>SMRKKIFKPEELRQALMPTLEALYRQDPESLPFRQPVDPQLLGIPDYFDIVKNPMDLSTIKRKLDTGQYQEPWQY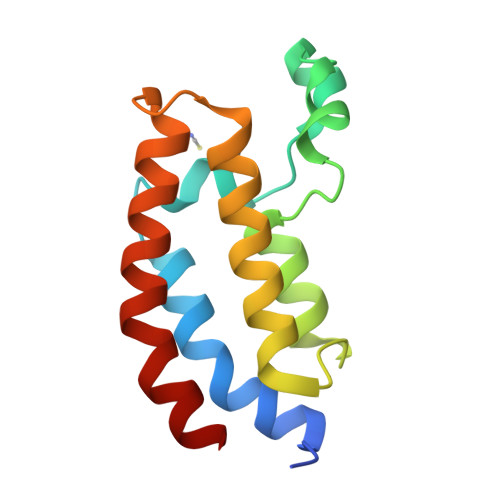VDDVWLMFNNAWLYNRKTSRVYKFCSKLAEVFEQEIDPVMQSLG[2x]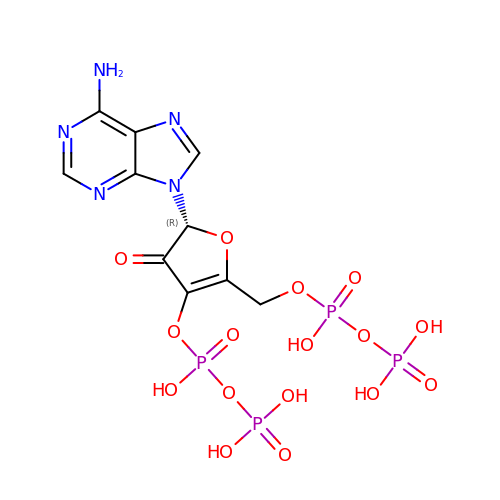(5R)-5-(6-amino-9H-purin-9-yl)-2-({[(S)-hydroxy(phosphonooxy)phosphoryl]oxy}methyl)-4-oxo-4,5-dihydrofuran-3-yl trihydrogen diphosphate | C10 H13 N5 O16 P4 | CDOGMROMDFBAJR-SNVBAGLBSA-N>[6x]GSHMPKRTFTKEDIRKFVEEENVRYLRLQFTDILGTIKNVEVPVSQLEKVLDNEMMFDGSSIEGFVRIEESDMYLHPDLDTWVIFPWTAGQGKVARLICDVYKTDGTPFEGDPRANLKRVLKEMEDLGFTDFNL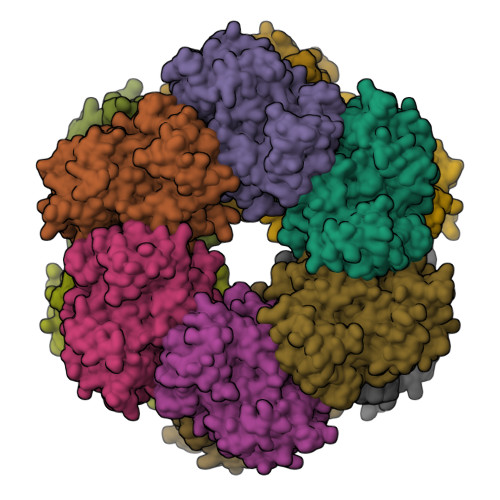GPEPEFFLFKLDEKGEPTLELNDDGGYFDLAPTDLGENCRRDIVLELEDMGFDIEASHHEVAPGQHEIDFKYADAVTACDNIQTFKLVVKTIARKHNLHATFMPKPLFGVNGSGMHFNVSLFKGKENAFFDPNTEMGLTETAYQFTAGVLKNARGFTAVCNPLVNSYKRLVPGYEAPCYIAWSGKNRSPLIRVPSSRGLSTRIEVRSVDPAANPYMALAAILEAGLDGIKNKLKVPEPVNQNIYEMNREEREAVGIQDLPSTLYTALKAMRENEVIKKALGNHIYNQFINSKSIEWDYYRTQVSEWERDQYMKQY> 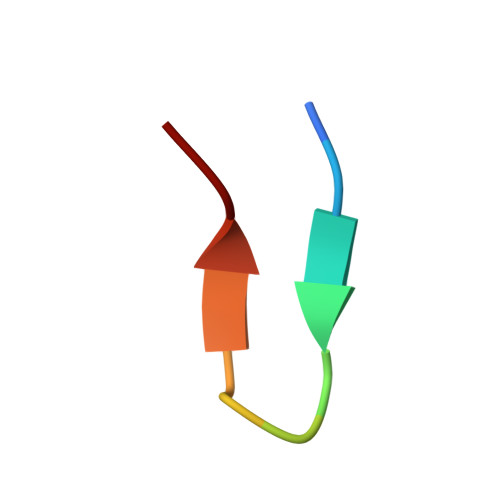WMLDPIAGKWSR Cofactor-independent urate oxidase (UOX) is an ∼137 kDa tetrameric enzyme essential for uric acid (UA) catabolism in many organisms. UA is first oxidized by O2 to de­hydro­isourate (DHU) via a peroxo intermediate. At different stages of the reaction both catalytic O2 and water occupy the ‘peroxo hole’ above the organic substrate. UOX belongs to a group of intriguing cofactor-independent oxidases and oxygenases that rely on their organic substrates for O2 activation.

Here, high-resolution neutron/X-ray crystallographic analysis at room temperature has been integrated with molecular dynamics simulations to investigate the hydration step of the reaction. To maximize the signal-to-noise ratio (S/N) of the neutron diffraction data we employed perdeuterated UOX (DUOX) instead of relying on protium (1H)/deuterium (2H or D) replacement of exchangeable hydrogens as done in previous studies on this system. The asymmetric unit contains a single DUOX chain that generates the biological tetramer of D2 symmetry following the application of crystallographic symmetry operations. W1O is hydrogen bonded to Thr57*DG1 at a distance of 2.16 Å. The visualization of W1 hydrogens allows us to also define an unanticipated O—H⋯π interaction with the ligand. Occupancy refinement for this atom gives a value of 0.78. In the final model the CA–CB–OG1–DG1 torsion angle displays a value of −110.4° resulting in a slight downward orientation of the OG1–DG1 bond towards the ligand plane with the deuteron at 2.77 Å from 8AZAN7, thus indicating another O—H⋯π interaction [Fig. 4(c)]. All deuterons bound to Lys10*NZ also refine to high occupancy (>0.90) with a hydrogen bond between Lys10*DZ1 and Thr57*OG1 at a distance of 1.97 Å. Taken together, experiment and theory (both standard MD and QM/MM-MD) are in excellent agreement and support the view that the minor crystallographic conformation favours the displacement of W1 from the peroxo hole.

> MSAVKAARYGKDNVRVYKVHKDEKTGVQTVYEMTVCVLLEGEIETSYTKADNSVIVATDSIKNTIYITAKQNPVTPPELFGSILGTHFIEKYNHIHAAHVNIVCHRWTRMDIDGKPHPHSFIRDSEEKRNVQVDVVEGKGIDIKSSLSGLTVLKSTNSQFWGFLRDEYTTLKETWDRILSTDVDATWQWKNFSGLQEVRSHVPKFDATWATAREVTLKTFAEDNSASVQATMYKMAEQILARQQLIETVEYSLPNKHYFEIDLSWHKGLQNTGKNAEVFAPQSDPNGLIKCTVGRSSLKSKL4-bromo-2,5-dimethoxyaniline | C8 H10 Br N O2 | 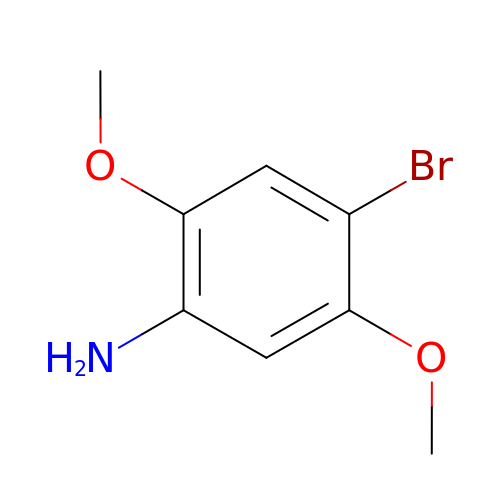YLONQFVJDASUEB-UHFFFAOYSA-N>MTHVEVVATITPQLYIEETLIQKINHRIDAIDVLELRIDQFENVTVDQVAEMITKLKVMQDSFKLLVTYRTKLQGGYGQFTNDSYLNLISDLANINGIDMIDIEWQADIDIEKHQRIITHLQQYNKEVIISHHNFESTPPL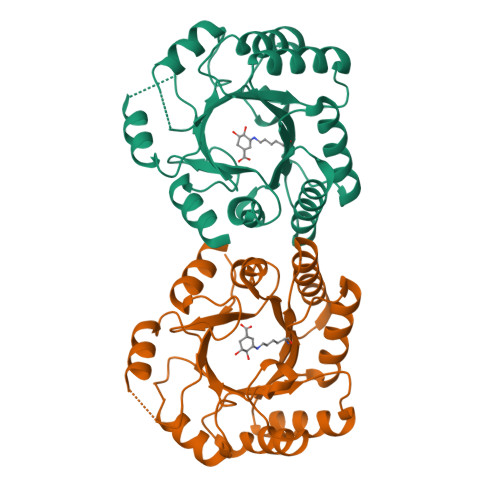DELQFIFFKMQKFNPEYVKLAVMPHNKNDVLNLLQAMSTFSDTMDCKVVGISMSKLGLISRTAQGVFGGALTYGCIGEPQAPGQIDVTDLKAQVTLY[2x]>[2x]SNAMNNELSPVALRQMSCAAGTTQTACTDDNALAYYNTTKGGR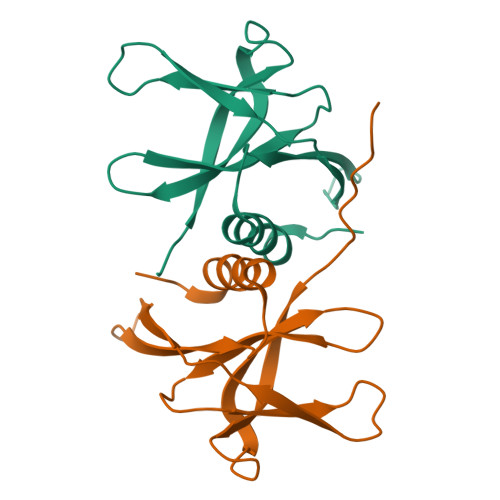FVLALLSDLQDLKWARFPKSDGTGTIYTELEPPCRFVTDTPKGPKVKYLYFIKGLNNLNRGMVLGSLAATVRLQ> SMALGPFPAMENQVLVIRIKIPNSGAVDWTVHSGPQLLFRDVLDVIGQVLPEATTTAFEYEDEDGDR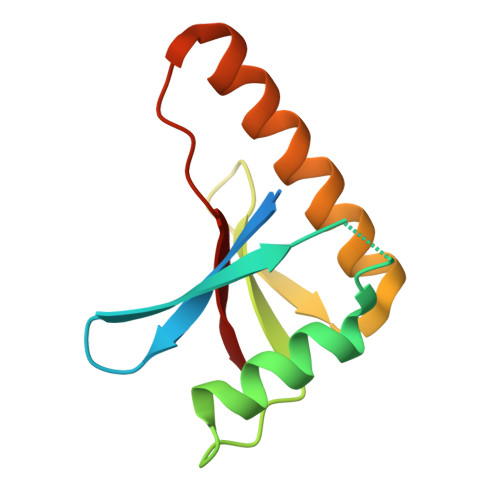ITVRSDEEMKAMLSYYYSTVMEQQVNGQLIEPLQIFPRA>[2x]QPQFNEDTLQQRLQALIESAGENWTYAIFWQISHDFDSSTGDNTV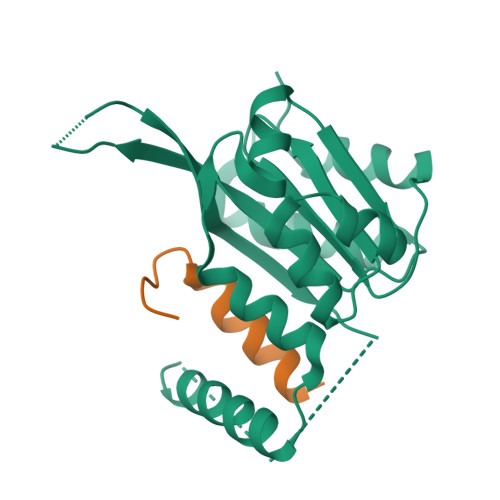ILGWGDGYYKGEEDKEKKKNNTNTAEQEHRKRVIRELNSLISGGIGVSDESNDEEVTDTEWFFLVSMTQSFVNGVGLPGESFLNSRVIWLSGSGALTGSGCERAGQGQIYGLKTMVCIATQNGVVELGSSEVISQSSDLMHKVNNLFNFN;>[2x]SSKKRCFKRSSSTSKLLNKVAARASSMGTILGASIEGTLISSTPLSSCL Here, we describe two novel OTU-like DUBs in Legionella – LotB (Lpg1621; Ceg23) and LotC (Lpg2529). Whereas the overall fold of the catalytic core of LotB and LotC resembles that of other OTU-DUBs, both showed apparent differences in the helical arm region, which has been shown to serve as an S1-binding site and interact with ubiquitin. The structure and sequence alignment with other OTUs clearly showed that both LotB and LotC contain a relatively long insertion between the Cys-loop and the variable loop, compared to other OTU members. Based on the catalytic cysteine and histidine residues of the two OTU domains on LotA, we analyzed the sequence and found that both OTU domains of LotA contain the extended insertion between the Cys loop and the variable loop (179 and 178 amino acids, respectively). Together, our results identify Lot-DUBs as a novel class of the OTU-family with longer insertions in the helical lobe region.

Consistent with the recent evidence, Lpg1621 exclusively processed the K63-linked Ub2, while Lpg2529 showed activity against K6-, K11-, K33-, K48-, and K63- linked Ub2. Based on the sequence analysis, we identified the conserved catalytic triad for both LotB (D27, C29, and H270) and LotC (D17, C24, and H304). While LotC retained its activity with the predicted OTU domain (7–310), LotB lost its activity after deletion of 50 amino acids (300–350) located at the C-terminus, beyond the predicted OTU domain (11–283). LotC lacks this S1’ site, causing the VME group between two ubiquitin moieties to be unable to reach the catalytic cysteine. In comparison, the helical lobes in LotB and LotC contain 183 and 210 amino acids, respectively. For LotC, we identified several hydrophobic interactions of the extended helical region (Tyr119 and Tyr149) with ubiquitin (Ile44). During the simulation, the C-terminus of ubiquitin (Arg72 and Arg74) formed transient electrostatic interactions with LotC (Glu153 and Glu245). Remarkably, a single mutation on E153 completely abolished the catalytic activity, which indicates that the electrostatic interactions are essential for the correct docking of the ubiquitin C-terminus into the catalytic pocket of LotC. The NEDD8, which has an alanine instead of Arg72 in ubiquitin, showed no modification toward LotC. By contrast, most of the enriched proteins from the inactive LotC pull-down were non-membrane-bound organelle- and ribosome-related proteins (RPS8, RPLP2, RPS27, RPLP1, and RPL13).

>FNVDNSGKGNCLYYAYSISLMYYLRAKNNVKITEDIFNKLGLKEEDRARLRKLLSKDPDRAFTRDEIKTIIEPILGRATRDLAAEHTKVEFKSSPHDTPLFSSLHYAVEFGFKRSLQINESELTLLIDNDFSNPDYTEAEIYKVSGLLDALQEYILTRTPSVIEEFNRQWENKKQELKEQSLTEKEIQVHQATILDNILRKETIDFLLAENEKHLDEYREHLRREFVWGSEETLMVLHRAIQGERMVRNHEGRIEPVYDHEIILHVHRNGASPSYQAGSPEMILNNEGNVHWTSIIP[2x]>MERYESLFAQLKERKEGAFVPFVTLGDLGIEQSLKIIDTLIEAGADALELGIPFSDPLADGPTIQNATLRAFAAGVTPAQCFEMLAIIREKHPTIPIGLLMYANLVFNKGIDEFYARCEKVGVDSVLVADVPVEESAPFRQAALRHNVAPIFICPPNADDDLLRQIASYGRGFTYLLSRAGVTGAENRAALPLNHLVAKLKEYNAAPPLQGFGISAPDQVKAAIDAGAAGAISGSAIVKIIEQHINEPEKMLAALKVFVQPMKAATRS[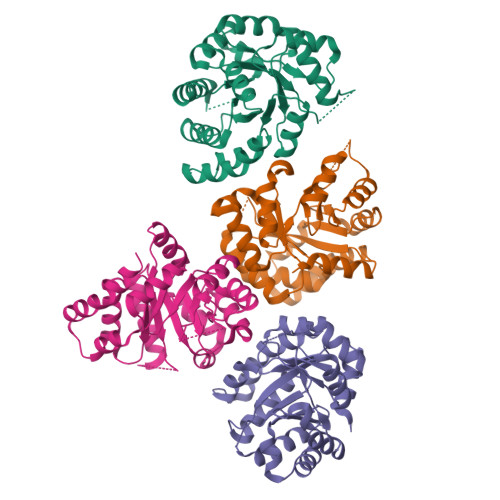2x]In common with all reported high-affinity binders, these peptides incorporate a signature p53-derived interacting motif comprising F, W and L residues that respectively dock into discrete hydrophobic pockets in the N-terminal domain of Mdm2. The Mdm2 and Mdm4 N-terminal domains that bind p53 share considerable structural homology, and there is significant interest in the clinical development of potent small molecule and peptidic dual inhibitors. The p53-degrading function of Mdm2 is enhanced by the structurally related paralog Mdm4 (also known as MdmX).

Towards reconciling this functional disparity, we have solved the structure of M011 bound to Mdm2 (residues 6–125). The crystal structure of M011 bound to Mdm2-M62A shows 2 unique complexes in the asymmetric unit. Within each, a single molecule of M011 interacts with a pronounced hydrophobic cleft that binds endogenous p53 (residues 19 to 26). As with other peptide antagonists, an interfacing signature triad of F19, W23 (6-chloro) and L26 residues (numbering based on p53 sequence) project their side chains into discrete apolar sub-pockets (“Phe”, “Trp” and “Leu” pockets). The structure highlights ready accommodation of the 6-chlorotryptophan chlorine atom by the hydrophobic pocket. Comparison with the structure of a similar stapled peptide (M06), comprising native tryptophan bound to the same Mdm2 construct shows remarkable similarity. Each M011 complex, from the asymmetric unit, shows high structural similarity to the corresponding complex bound to M06 (all-atom derived RMSDs = 0.167 and 0.126 Å). The major difference arises from rotation around the CHI1 bond of the L57 side chain in Mdm2 to widen the Trp pocket, with other residues comprising this pocket (F86, F91, I99) remaining unchanged. This optimal formation of Van der Waals contacts around the 6-chloro moiety, resulting from the change in conformation of L59, explains the ~8-fold increased binding affinity of M011 over the parental stapled peptide lacking the 6-chloro modification (PM2). Structural differences are also observed in the lid/hinge region between the two M011: Mdm2 complexes in the asymmetric unit.

>GPMSVPTDGAVTTSQIPASEQETLVRPKPLLLKLLKSVGAQKDTYTMKEVLFYLGQYIATKRLYDEKQQHIVYCSNDLLGDLFGVPSFSVKEHRKIYTMIYRNLVVVNQQESSDSGTSVSEN[2x];>[2x]TSFXEYWALLLX> MSLYRRLVLLSCLSWPLAGFSATALTNLVAEPFAKLEQDFGGSIGVYAMDTGSGATVSYRAEERFPLCSSFKGFLAAAVLARSQQQAGLLDTPIRYGKNALVPWSPISEKYLTTGMTVAELSAAAVQYSDNAAANLLLKELGGPAGLTAFMRSIGDTTFRLDRWELELASAIPGDARDTSSPRAVTESLQKLTLGSALAAPQRQQFVDWLKGNTTGNHRIRAAVPADWAVGDKTGTCGVYGTANDYAVVWPTGRAPIVLAVYTRAPNKDDKHSEAVIAAAARLALEGLGVNGQ

Class A β-lactamases, including KPC-2, hydrolyze the amide bond in β-lactam antibiotics through sequential acylation and deacylation steps. The catalytic Ser70 residue attacks the carbonyl carbon of the β-lactam resulting in cleavage of the amide bond and formation of a covalent acyl-enzyme intermediate. Subsequently, Glu166 activates a catalytic water molecule for attack on the carbonyl carbon of the acyl-enzyme leading to hydrolysis of the ester bond between Ser70 and the drug. However, the emergence of the KPC-2 carbapenemase has resulted in widespread resistance to these drugs, suggesting it operates more efficiently.

To further investigate the role of Asn170 in penicillin and carbapenem hydrolysis, we determined the X-ray structure of the KPC-2 N170A apoenzyme as well as product complexes with ampicillin and imipenem. The structure of the N170A apoenzyme is very similar to that of the wildtype KPC-2 apoenzyme with the only major difference being the smaller alanine side chain at position 170, which creates a pocket not found in wildtype and thus expands the volume of the active site in this region. Asn170 along with Glu166 coordinates the hydrolytic water molecule critical for the deacylation reaction. Since sharply decreased values of both kcat and KM are consistent with impaired deacylation in the β-lactamase kinetic scheme, we hypothesized that the N170A substitution results in a decreased rate of deacylation of the carbapenem substrates. To test this hypothesis, single turnover kinetics were performed for the N170A enzyme with imipenem, revealing a modest 5-fold decrease in the acylation rate (k2) but a 2800-fold decrease in the deacylation rate (k3) as compared with wildtype KPC-2 such that deacylation is strongly rate limiting for imipenem hydrolysis in the mutant. Based on this evidence, we speculate that the impaired deacylation of imipenem observed with the KPC-2 N170A enzyme is due to the C6-hydroxyethyl side chain occupying the cavity created by the substitution and displacing the catalytic water molecule.The Ets transcription factor family consists of 28 genes in humans containing the evolutionarily conserved 85 amino acid Ets DNA-binding domain, originally identified as a viral oncogene (E26 transformation-specific). The Ets domain is a variant helix-turn-helix (winged helix) structure, comprising three α-helices and a four-stranded antiparallel β-sheet. Here, we present the crystal structures of the Ets domains of the entire PEA3 subfamily (Etv1, Etv4, and Etv5) together with the structure of the Erg family member (Fev). Furthermore, a new Ets dimerization interface linked by a redox-sensitive disulfide bond is identified, and this dimerization is shown to result in a significant inhibition of DNA binding, potentially linking Ets transcription factors with cellular redox regulatory mechanisms.

In the DNA complex structures of Etv5 and Fev (which are determined to 1.9 and 2.0 Å resolution, respectively), we observe a network of coordinated water molecules contributing to sequence recognition upstream to the GGA core. From analysis of the high resolution structures of the Etv5 and Fev DNA complexes (which are high enough resolution (< 2.0 Å) to reliably locate ordered waters), a number of additional contacts can be seen, which appear to enable direct readout of additional base pairs both upstream and downstream of the GGA core. The two C-G base pairs at positions −2 and −1 lie close to a highly coordinated network of four water molecules conserved in both structures and are coordinated by polar contacts to the side chains of Asp-387 (Fev Asp-99), Ser-390 (Fev Ser-102), Arg-394 (Fev Arg-106), Tyr-412 (Fev Tyr-124), and the phosphate oxygens of the two cytosine nucleotides at positions −2 and −1. The requirement in this network for the water closest to the base at position −1 to be a hydrogen bond acceptor almost perfectly explains the observed sequence preferences at this position, with a strong selection of cytosine (∼75% occurrence) and the only other allowed base being adenine (∼15% occurrence), which is also able to donate a hydrogen bond, although in this case the hydrogen bonding distance would be significantly longer (≈4.0 Å). In the Etv5 and Fev DNA complex structures, the corresponding residue (Etv5-Tyr-428 and Fev-Tyr-107, respectively) can be seen to occupy two conformations, one in which the two interactions detailed above are conserved, and an additional conformation where the side chain hydroxyl lies close to Etv5-Lys-432/Fev-Lys-111 and provides a large contact surface, with the potential for favorable van der Waals interactions to bases at positions +5 and +6 on the complementary strand. The finding that both conformations of this residue appear to occur together indicates that the dynamic nature of the side chains of the recognition helix may be even more important for DNA recognition than previously thought.

> SMKGSGQIQLWQFLLELLADRANAGCIAWEGGHGEFKLTDPDEVARRWGERKSKPNMNYDKLSRALRYYYDKNIMSKVHGKRYAYRFDFQGLAQACQPPPAH Anion exchanger 1 (AE1, band 3) is a major membrane protein of red blood cells and plays a key role in acid-base homeostasis, urine acidification, red blood cell shape regulation, and removal of carbon dioxide during respiration. AE1, a member of the solute carrier ion transport family 4 (SLC4), mediates the exchange of HCO3− with Cl− across plasma membranes. Mammalian erythrocyte AE1 is a ~100 kD integral transmembrane glycoprotein consisting of an N-terminal cytoplasmic domain (CD, residues 1 to 360 in human AE1) and a C-terminal trans-membrane domain (TMD, residues 361 to 911 in human AE1). Here we present the cryoEM structures of full-length bovine AE1 with its TMD captured in both IF and OF conformations.

3D classification using the C1 symmetry resulted in three major classes that differ mostly in the position of the CD. Two classes showed fully connected CD and partially connected CD respectively. 3D refinement of these two classes yielded 3D reconstructions at a resolution of 6.3 Å and 6.9 Å respectively. The overall size and shape of these reconstructions suggest unambiguously that they are dimers of full-length AE1, each with a PMAL-C8 buried TMD and an associated CD. Both the TMD and CD dimers have an elongated shape. The limited direct contact between the TMD and the CD leads to a large corridor between the two domains, providing an unobstructed access for the substrate ions to the intracellular side of the TMD. We have previously demonstrated that there is a flexible linker between CD and TMD in the AE1 monomer that may play a significant role in the red blood cell elasticity, providing a mechanism to connect the cytoskeleton (given that AE1 CD binds various cytoplasmic proteins) with the red blood cell membrane.

>[4x]MGDPEEYEDQLEETLEQKEYEDHDSVSIPMEEAEGDTIQEEEAEARVNQLTDTDYHTTSQHPETHKVCVQLRELVMDEKNQEIQWMETARWVGLEENLGKDGIWGRPHLPYLNFWSLLELQKAFAKGTVLLDLPGKSLAEVANQLLDRFTFEGQIQPDDQDNLLRVLLLKHSHASDMEALGGVKPVVVTHSGDPSEPLLPQHPSLETELFCEQGEGSTRGHAPEILGKSPQDWEATLVLVGCARFLKRPVLGFVRLKEPMEPEPKPEGSEEPAVPVRFLIVLLGPEGPNINYTQLGRAAATLMSERVFWNDAYLAQSKETLVQSLEGFLDCSLVLPPLDAPSEKALLSLVPVQKELLRRRYLPSPAKPDPSIFKDLDVKKGPGDTPEDPLQRTGKLFGGLVRDIRRRYPRYLSDITDALSPQVLSAIIFIYFAALTPAITFGGLLGDKTENMIGVSELLLSTALQGIIFSLLGAQPLLVLGFSGPLLVFEEAFYSFCQTNNLEYIVGRVWIGFWLILLVVLVVAFEGSFLVRFISRYTQEIFSFLISLIFIYETFYKLVTIFQDHPLQKNYDHDVLTTPKPQAALPNTALLSLVLMAGTFFLAMMLRKFKNSSYFPGKLRRIIGDFGVPISILIMVMVDALIQDTYTQKLSVPEGLSVSNPTERDWLIHPLGIRVEFPIWMMFASALPALLVFILIFLESQITTLIISKPERKMVKGSGFHLDLLLIIGMGGVGAIFGMPWLSATTVRTVTHANALTVMSKDSTPGAVSQIQGVKEQRISGLLVAVLVGVSILMGPVLRHIPLAVLFGIFLYMGVTSLSGIQLFDRVLLLLKPRKYYPEVPYARRVKTWRMHLFTITQIVCLVVLWVVRSIKQISLALPFILILTVPLRRFLLPFIFRDMELKLLDADDVKLNLDEQNGQDEYDEVAMPV>SNAMAEDKGRKVVVSALQFACTDDVSTNVTTAERLVRAAHKQGANIVLIQELFEGYYFCQAQREDFIQRAKPYKDHPTIMRLQKLAKELGVVIPVSFFEEANNAHYNSIAIIDADGTDLGIYRKSHIPDGPGYEEKFYFNPGDTGFKVFQTKYAKIGVAICWDQWFPEAARAMALQGAEILFYPTAIGSEPHDQSIDSRDHWKRVMQGHAGANLVPLVASNRIGNEIIETEHGKSEIKFYGNSFIAGPTGEIVSIADDKEEAVLIAEFNLDKIKSMRHCWGVFRDRRPDLYKVLLTLDGKNPVL[16x]

The arginine route involves three enzymatic steps: (i) arginine decarboxylation to agmatine by arginine decarboxylase (ADC, EC 4.1.1.19); (ii) deimination of agmatine by agmatine iminohydrolase (AIH, EC 3.5.3.12) and (iii) hydrolysis of N-carbamoylputrescine (NCP) to putrescine by N-carbamoylputrescine amidohydrolase (CPA, EC 3.5.1.53), with the release of carbon dioxide and ammonia. N-carbamoylputrescine amidohydrolase enzymes belong to nitrilases, and more precisely, to C-N hydrolases breaking non-peptide bonds using Cys-Glu-Lys catalytic triad. The octameric MtCPA enzyme is assembled into an incomplete helical twist, made by four tight dimers with swapped C-termini. As in other nitrilases, the substrate hydrolysis is carried out by the catalytic triad, composed in MtCPA of Glu48 (proton acceptor), Lys121 (proton donor) and Cys158 (nucleophile).

The structures of wild-type MtCPA, crystallized in the presence of PUT and CAD in the solution, were determined at 1.97 and 2.19 Å resolution, respectively. Inspection of the electron density maps, representing the structure of MtCPA cocrystallized with PUT, brought unexpected, but very informative results. Instead of linear PUT, the reaction intermediate, DHMP, was observed in the active site. More interestingly, DHMP was covalently bound to the catalytic Cys158. The DHMP covalent adduct is stabilized by placement of one of its oxygen atoms within the oxyanion hole, created by Nζ of Lys121 and the backbone N of Trp159 (see Active Site and the Reaction Mechanism). DHMP adduct was most probably formed as the result of the reaction of the amine group of PUT with carbon dioxide, absorbed by the crystallization drop, followed by nucleophilic attack of the active Cys158. This showed that the oxyanion hole, next to the MtCPA catalytic triad, is able to stabilize the otherwise labile geminal diol. Subsequently, the amino group of the intermediate accepts a proton, donated by Glu48, and leaves as the first by-product, ammonia, resulting in the planar S-acyl intermediate-enzyme complex, which is hydrated to yield the tetrahedral oxyanionic geminal diol (present in the crystal structure of MtCPA/DHMP complex). All bound amines, CAD, PUT and DHMP, present the same hydrogen bond between terminal amine group and the side chain oxygen of Glu187.Galectin (Gal) is a lectin that binds to β-galactosides. Because the primary and tertiary structures of Gal-13 are highly conserved among all galectins, it had been named galectin-13. However, our crystallographic and biochemical experiments (solid phase experiment, hemagglutination assay, and biolayer interferometry) proved that wild-type Gal-13 could not bind lactose or a rhamnogalacturonan Ι domain (RG-I-4) from Ginseng Pectin. Primary structure alignment showed that a highly conserved histidine residue was modified to arginine (Arg53) in the ligand binding site of wild-type Gal-13, which may be why Gal-13 could not bind lactose.

We assumed that mutation of Arg53 to histidine would be sufficient to recover the ability of Gal-13 to bind lactose. However, this was not the case, and R53H did not co-crystallize with lactose. In the present study, we used PEG400 as the cryoprotectant for R53H crystal, and not glycerol. Surprisingly, we found a different compound bound in the ligand binding site of R53H. Mass spectroscopy identifies this compound as Tris. However, here, lactose could not co-crystallize with R53H, but Tris could. Tris has three hydroxyl groups and binds in a triangular shape. It seems that Arg55 plays a role in stabilizing Tris in R53H. Here, we found two Gal-13 variants (R53H and R53HR55N) that could co-crystallize with Tris, that also has three hydroxyl groups and shows a triangular shape when bound in the ligand binding site. However, the hydroxyl groups from Tris could not be merged with the oxygen atoms of lactose.

> GSHMSSLPVPYKLPVSLSVGSCVIIKGTPIHSFINDPQLQVDFYTDMDEDSDIAFHFRVHFGNHVVMNRREFGIWMLEETTDYVPFEDGKQFELCIYVHYNEYEIKVNGIRIYGFVHRIPPSFVKMVQVSRDISLTSVCVCN> GAMVIEKEDVETNASNGQRVDLSSELDKLKKLENATVHMEFKPDAKAPAFYNLFSVSSATKKDEYFTMAVYNNTATLEGRGSDGKQFYNNYNDAPLKVKPGQWNSVTFTVEKPTAELPKGRVRLYVNGVLSRTSLRSGNFIKDMPDVTHVQIGATKRANNTVWGSNLQIRNLTVYNRALTPEEVQKRS

Streptococcus pneumoniae Neuraminidase A (NanA) is a multi-domain protein anchored to the bacterial surface. Upstream of the catalytic domain of NanA is a domain that conforms to the sialic acid-recognising CBM40 family of the CAZY (carbohydrate-active enzymes) database. This domain has been identified to play a critical role in allowing the bacterium to promote adhesion and invasion of human brain microvascular endothelial cells, and hence may play a key role in promoting bacterial meningitis. Here we describe the crystal structure of the S. pneumoniae NanA CBM40 domain, hereafter named SpCBM.

Crystal structures of SpCBM, complexed with α2,3-sialyllactose (Neu5Ac-α2,3-Gal-β1,4-Glc, from here on referred to as 3’SL) and α2,6-sialyllactose (Neu5Ac-α2,6-Gal-β1,4-Glc, from here on referred to as 6’SL) are also described. For the complexed structures, both 3’SL and 6’SL were co-crystallized with SpCBM. There are no significant conformational changes between the apo SpCBM structure and the complexed structure, and superimposition of the apo and holo structures gives an RMSD of 0.48 Å over all Cα atoms for both 3’SL and 6’SL. In the 3’SL and 6’SL complexes, the protein structures are highly similar, giving an RMSD of 0.06 Å for all of the Cα atoms while the sialic acid moieties of the ligands are completely superimposable. The lactose moieties of the 3’SL and 6’SL, however, point in opposite directions. In 6’SL, glucose O6 interacts with the side chain of Asp180. The carboxylate group of Neu5Ac forms a bidentate interaction with Arg274, a common feature in proteins that bind sialic acid. Other Neu5Ac atoms make additional interactions with SpCBM: O4 interacts with the side chain of Glu195 as does the N5 of the acetamido group; the O10 carbonyl oxygen of the acetamido group interacts with Asn209; the glycerol O8 hydroxyl oxygen interacts with the imidazole nitrogen of Trp280. Phe167 provides a hydrophobic platform supporting the glycerol carbons (C7 to C9) that are ~4 Å away, and also forms part of the hydrophobic pocket accommodating the acetamido methyl group. A striking feature of the protein is a deep, negatively charged cavity adjacent to the sialic acid binding site. This pocket is formed by four residues (Glu195, Gln203, Asn207 and Asn209), and is occupied by a lysine from a symmetry-related molecule.> MEQNLFALSLDDTSSVRGSLLDTKFAQTRVLLSKAMAGGDVLLDEYLYDVVNGQDFRATVAFLRTHVITGKIKVTATTNISDNSGCCLMLAINSGVRGKYSTDVYTICSQDSMTWNPGCKKNFSFTFNPNPCGDSWSAEMISRSRVRMTVICVSGWTLSPTTDVIAKLDWSIVNEKCEPTIYHLADCQNWLPLNRWMGKLTFPQGVTSEVRRMPLSIGGGAGATQAFLANMPNSWISMWRYFRGELHFEVTKMSSPYIKATVTFLIAFGNLSDAFGFYESFPHRIVQFAEVEEKCTLVFSQQEFVTAWSTQVNPRTTLEADGCPYLYAIIHDSTTGTISGDFNLGVKLVGIKDFCGIGSNPGIDGSRLL;> GPVCAEASDVYSPCMIASTPPAPFSDVTAVTFDLINGKITPVGDDNWNTHIYNPPIMNV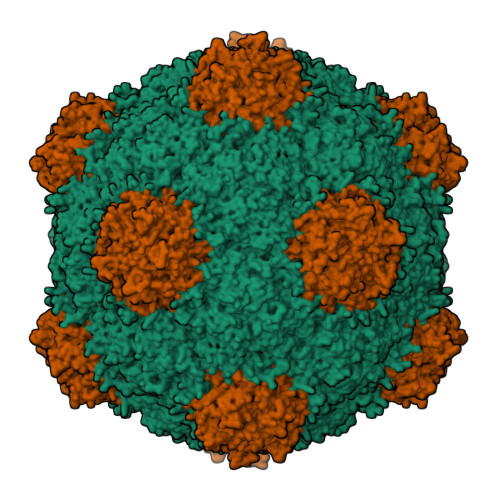LRTAAWKSGTIHVQLNVRGAGVKRADWDGQVFVYLRQSMNPESYDARTFVISQPGSAMLNFSFDIIGPNSGFEFAESPWANQTTWYLECVATNPRQIQQFEVNMRFDPNFRVAGNILMPPFPLSTETPPL> GSMADEATRRVVS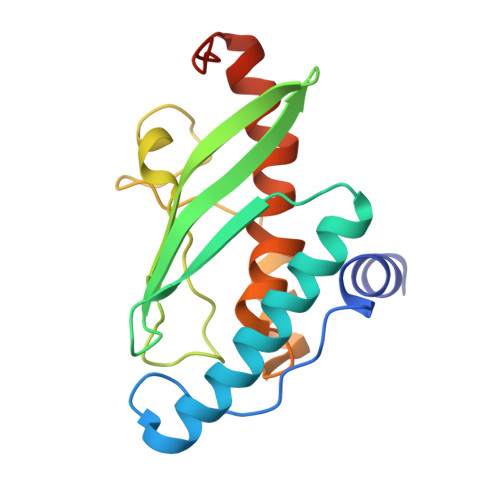EIPVLKTNAGPRDRELWVQRLKEEYQSLIRYVENNKNADNDWFRLESNKEGTRWFGKCWYIHDLLKYEFDIEFDIPITYPTTAPEIAVPELDGKTARMYRGGKICLTDHFKPLWARNVPKFGLAHLMALGLGPWLAVEIPDLIQKGVIHHKEKCNQ>VERYSLSPMKDLWTEEAKYRRWLEVELAVTRAYEELGMIPKGVTERIRNNAKIDVELFKKIEEKTNHDVVAFVEGIGSMIGEDSRFFHYGLTSSDVLDTANSLALVEAGKILLESLKEFCDVLWEVANRYKHTPTIGRTHGVHAEPTSFGLKVLGWYSEMKRNVQRLERAIEEVSYGKISGAVGNYANVPPEVEEKALSYLGLKPEPVSTQVVPRDRHAFYLSTLAIVAAGIERIAVEIRHLQRTEVLEVEEPFRKGQRGSSAMPHKKNPITCERLTGLSRMMRAYVDPSLENIALWHERDISHSSVERYVFPDATQTLYYMIVTATNVVRNMKVNEERMKKNIDLTKGLVFSQRVLLKLIEKGLTRKEAYD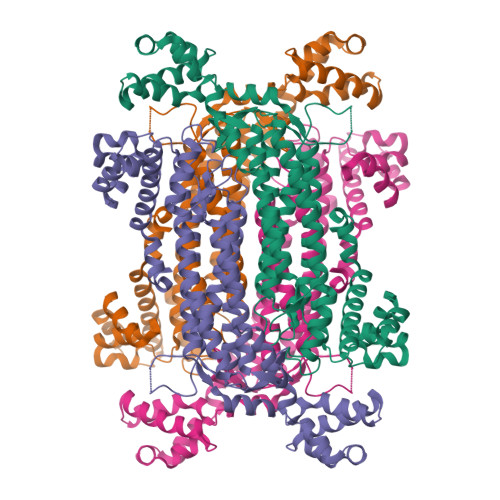IVQRNALKTWNSEKHFLEYLLEDEEVKKLVTKEELEELFDISYYLKHVDHIFERFEK[2x]> SNAMALSKSMHARNRYKDKPPDFAYLASKYPDFKQHVQINLNGRVSLNFKDPEAVRALTCTLLREDFGLSIDIPLERLIPTVPLRLNYIHWVEDLIGHQDSDKSTLRRGIDIGTGASCIYPLLGATLNGWYFLATEVDDMCFNYAKKNVEQNNLSDLIKVVKVPQKTLLMDALKEESEIIYDFCMCNPPFFANQLEAKGVNSRNPRRPPPSSVNTGGITEIMAEGGELEFVKRIIHDSLQLKKRLR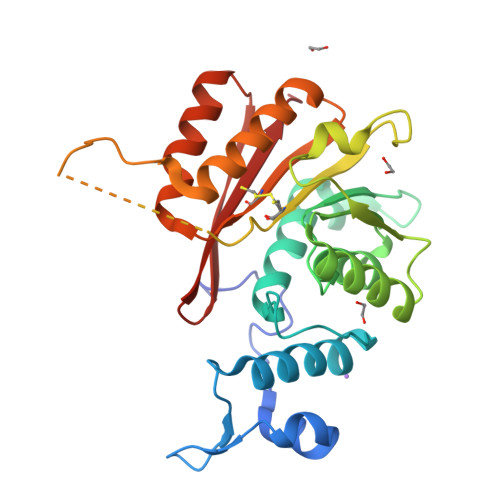WYSCMLGKKCSLAPLKEELRIQGVPKVTYTEFCQGRTMRWALAWSFYD>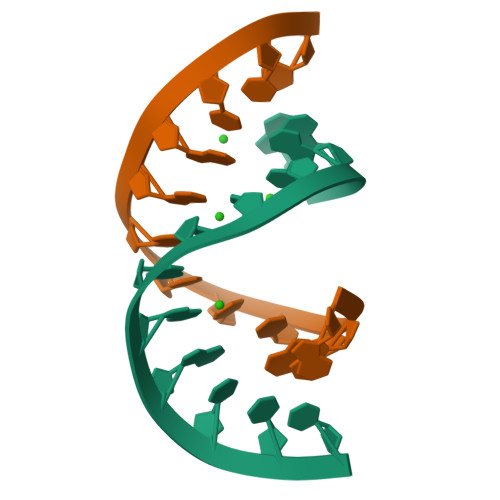[4x]GGGCCCGGACCC>NLQSQFFIEHILQILPHRYPMLLVDRITELQANQKIVAYKNITFNEDVFNGHFPNKPIFPGVLIVEGMAQSGGFLAFTSLWGFDPEIAKTKIVAFMTIDKVKFRIPVTPGDRLEYHLEVLKHKGMIWQV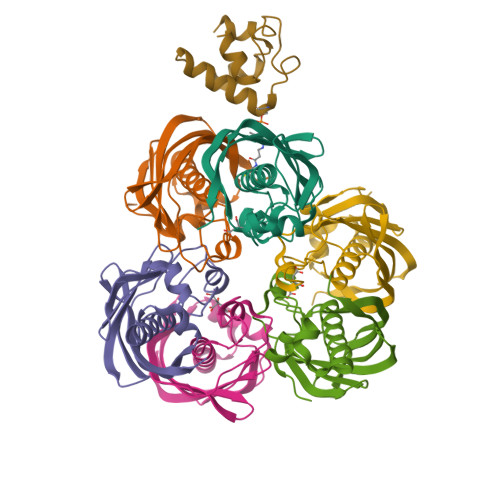GGTAQVDGKVVAEAELKAMIAERE[6x];> IQAVIAEQLNVDAAQVTPEAEFVKDLGADSLDVVELIMALEEKFGIEIPDEQAEKIVNVGDVVKY> MVNNNRPRRQRAQRVVVTTTQTAPVPQQNVPRNGRRRRNRTRRNRRRVRGMNMAALTRLSQPGLAFLKCAFAPPDFNTDPGKGIPDRFEGKVVSRKDVLNQSISFTAGQDTFILIAPTPGVAYWSASVPAGTFPTSATTFNPVNYPGFTSMFGTTSTSRSDQVSSFRYASMNVGIYPTSNLM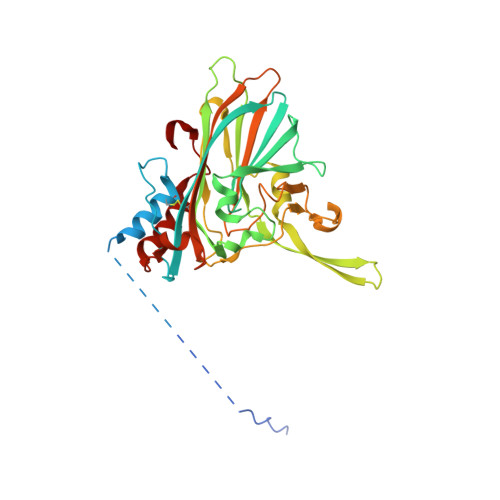QFAGSITVWKCPVKLSTVQFPVATDPATSSLVHTLVGLDGVLAVGPDNFSESFIKGVFSQSACNEPDFEFNDILEGIQTLPPANVSLGSTGQPFTMDSGAEATSGVVGWGNMDTIVIRVSAPEGAVNSAILKAWSCIEYRPNPNAMLYQFGHDSPPLDEVALQEYRTVARSLPVAVIAAQN>GPMGKPARKGCEWKRFLKNNWVLLSTVAAVVLGITTGVLVREHSNLSTLEKFYFAFPGEILMRMLKLIILPLIISSMITGVAALDSNVSGKIGLRAVVYYFCTTLIAVILGIVLVVSIKPGVTQKVGEIARTGSTPEVSTVDAMLDLIRNMFPENLVQACFQQYKTKREEVKPPSDPEMTMTEESFTAVMTTAISKTKTKEYKIVGMYSDGINVLGLIVFCLVFGLVIGKMGEKGQILVDFFNALSDATMKIVQIIMCYMPLGILFLIAGKIIEVEDWEIFRKLGLYMATVLTGLAIHSIVILPLIYFIVVRKNPFRFAMGMAQALLTALMISSSSATLPVTFRCAEENNQVDKRITRFVLPVGATINMDGTALYEAVAAVFIAQLNDLDLGIGQIITISITATSASIGAAGVPQAGLVTMVIVLSAVGLPAEDVTLII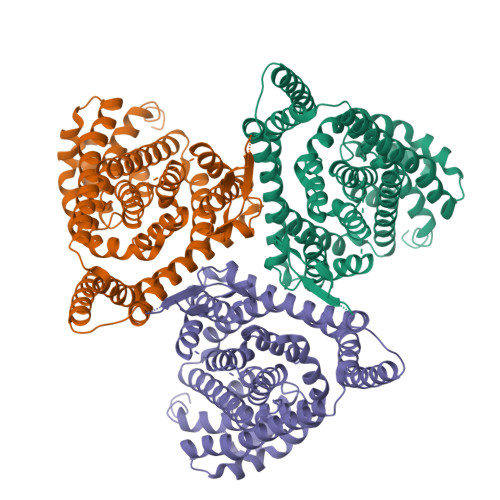AVDWLLDRFRTMVNVLGDAFGTGIVEKLSKKELEQMDVSSEVNIVNPFALESTILDNEDSDTKKSYVNGGFAVDKSDTISFTQTSQF[3x]> MSTKEDARSTCEKAARKAAESNDEEVAKQAAKDCLEVAKQAGMPTKEAARSFCEAAARAAAESNDEEVAKIAAKACLEVAKQAGMPTKEAARSFCEAA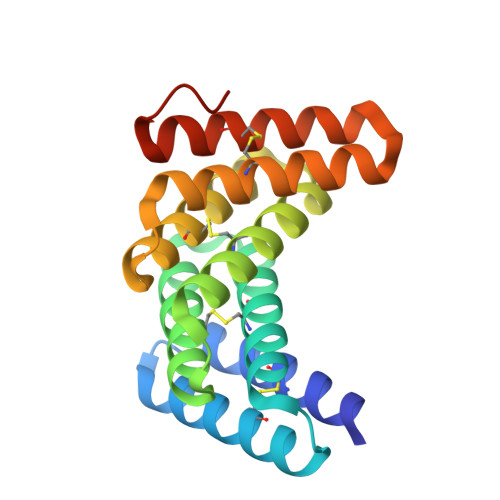ARAAAESNDEEVAKIAAKACLEVAKQAGMPTKEAARSFCEAAKRAAKESNDEEVEKIAKKACKEVAKQAGMPWLEHHHHHH>[2x]GPLGSKIVRIEKARDIPLGATVRNEMDSVIISRIVKGGAAEKSGLLHEGDEVLEINGIEIRGKDVNEVFDLLSDMHGTLTFVLIPSQ;>[2x]EGVPDLLV

PALS1 regulates cell polarity through binding to the PDZ-binding domain (PBM) of CRB3 with loss of PALS1 leading to disruption of cell polarity including loss of integrity of tight and adherens junctions. Importantly, the SARS-CoV-1 E protein’s PDZ-binding motif13 sequence allows interaction with the host cell polarity signalling protein PALS1 (Protein associated with Lin7/MPP5) thus interfering with epithelial function and integrity, a property of the SARS-CoV-1 E protein which is thought to be important for its virulence. As previously shown the PALS1 PDZ domains adopts a compact globular fold comprising five to six β‐strands and two α‐helices that form a β‐sandwich structure. Examination of both the PALS1 PDZ:SARS-CoV-1_E and PALS1 PDZ:SARS-CoV-2_E complexes showed that the E protein PBM peptides are bound in the canonical ligand-binding groove formed by the β2 strand and helix α2.

To understand the structural basis of the PALS1 PDZ and SARS-CoV-1/2 E PBM interaction, we determined the crystal structures of PALS1 PDZ bound to the SARS-CoV-1_E (SRVPDLLV) and SARS-CoV-2_E (EGVPDLLV) PBM peptides to resolutions of 1.74 and 1.9 Å, respectively. PALS1 PDZ:SARS-CoV-1_E and PALS1 PDZ:SARS-CoV-2_E superimposed with one another yielded an overall root‐mean‐square deviation (RMSD) of 0.72 Å. In the PALS1 PDZ:SARS-CoV-1_E complex, SARS-CoV-1_E Val75 is docked in the conserved hydrophobic pocket formed by PALS1 PDZ Leu267, Gly268 and Ala269. In addition, two hydrogen bonds are formed by Val271PALS PDZ –Leu74SARS-CoV-1_E located at the second β‐sheet of PALS1 PDZ. Lastly, an ionic interaction is found between Arg272PALS1 PDZ –Asp73SARS-CoV-1_E, and SARS-CoV-2_E Val75, Leu74 and Leu 73 are involved in hydrophobic interactions. Major differences are found among the hydrophobic contacts, with the rotamer of SARS-CoV-1_E Leu73 differing from SARS-CoV-2_E Leu74. Furthermore, in SARS-CoV-1_E only Val75, Leu74 and Leu 73 are involved in hydrophobic contacts, whereas in SARS-CoV-2_E Pro72, Val71 are also involved in hydrophobic contacts. A comparison of our structures with apo-PALS1 PDZ reveals that similarly, both SARS-CoV-1_E and SARS-CoV-2_E binding to PALS1 PDZ trigger rotation of PALS1 Phe318 out of the ligand-binding groove to allow binding of SARS-CoV-1/2_E PBM. Our ITC measurements revealed that whilst PALS1 PDZ did not bind to MERS-CoV_E, it bound to SARS-CoV-1_E with an affinity of 29.6 μM, and SARS-CoV-2_E with an affinity of 22.8 μM. However, despite the sequence differences between SARS-CoV-1_E and SARS-CoV-2_E PBM in positions −5 and −6, affinities for PALS1 PDZ are comparable, indicating that positions 0, −1, −2 and −3 are required for CoV_E PBM interaction with PALS1 PDZ and define binding, whereas positions −4, −5, −6 and −8 do not play a major role.>[3x]MAANSTRRPIIAFMSDLGTTDDSVAQCKGLMYSICPDVTVVDVCHSMTPWDVEEGARYIVDLPRFFPEGTVFATTTYPATGTTTRSVAVRIKQAAKGGARGQWAGSGAGFERAEGSYIYIAPNNGLLTTVLEEHGYLEAYEVTSPKVIPEQPEPTFYSREMVAIPSAHLAAGFPLSEVGRPLEDH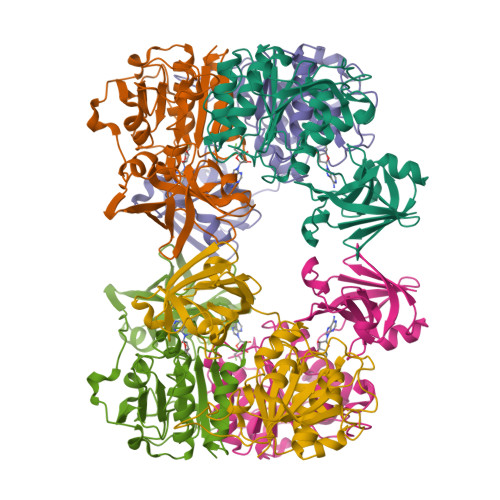EIVRFNRPAVEQDGEALVGVVSAIDHPFGNVWTNIHRTDLEKAGIGYGARLRLTLDGVLPFEAPLTPTFADAGEIGNIAIYLNSRGYLSIARNAASLAYPYHLKEGMSARVEAR Panoptes is a two-gene operon, optSE, wherein OptS is predicted to synthesize a nucleotide-derived second messenger and OptE is predicted to bind that signal and drive effector-mediated defence. Crystal structures show that OptS is a minimal CRISPR polymerase (mCpol) domain, a version of the polymerase domain found in type III CRISPR systems (Cas10). OptS constitutively synthesizes 2′,3′-c-di-AMP and other cyclic dinucleotides to hold OptE in an inactive state. During phage infection, Acb2 or similar immune evasion proteins are produced that sequester the OptS-derived signalling molecule, leading to a population of OptE that is no longer bound to cyclic dinucleotide and is free to become activated, in turn disrupting the bacterial membrane and resulting in phage defence.

We determined a 2.42 Å crystal structure of KpOptS bound to the ATP substrate analogue α,β-methyleneadenosine-5′-triphosphate (ApCpp). Our data showed four independent ligand binding sites; however, inconsistent occupancy for the ribose and adenine nucleobase led us to confidently model only one complete ApCpp and three molecules of pCpp. In the binding site, we find that the ribose from ApCpp and the α-phosphate of an adjacently bound ligand are poised for reaction within a distance of about 4–5 Å of each other. All ligands are stably bound to their respective protomers by means of divalent cations, here modelled as magnesium ions, which coordinate the triphosphate tail of the substrate. The metals are held in place as anticipated by active site aspartates D6 and D57, previously shown to be critical for complete catalytic activity. The binding pocket consists of amino acid contributions from two protomers, with the triphosphate bound to one protomer and the ribose and nucleobase positioned in an adjacent protomer, similar to what has been observed for ATP binding to Csm1 (Cas10). In the crystal structure, the adenine N-6 amino group is oriented towards an asparagine residue (N34) that is conserved between Kp and VnOptS. The only observed contact that was predicted to differ in amino acid identity between the two proteins was S30 (N31 in VnOptS). For the KpOptS S30N mutant, there was a nearly complete inversion of the ratio of 2′,3′-c-di-AMP relative to 3′,2′-cGAMP produced in a reaction containing only ATP and GTP. Although more subtle, the corresponding mutant of VnOptS (N31S) produced an increased proportion of 2′,3′-c-di-AMP and a decreased proportion of 3′,2′-cGAMP, relative to the wild type. These results agree with prior studies on Cas10 and GGDEF proteins highlighting the role of serine and asparagine amino acid recognition of adenine and guanine bases, respectively.

>[4x]MGSSHHHHHHGSMYIAIDGDDVGRKITSSYLSNSEERLTYISNKLNDTTKKISKMLLSNGFEIIFQAADGVTAKTDNEVNLNFVFDKIKSYSFDEITFSAGVGANLREAYVALLNSKSNGKNMISIYKDIL> MSFTNATFSQVLDDLSARFILNLPAEEQSSVERLCFQIEQAHWFYEDFIRAQNDQLPSLGLRVFSAKLFAHCPLLWKWSKVHEEAFDDFLRYKTRIPVRGAIMLDMSMQQCVLVKGWKASSGWGFPKGKIDKDESDVDCAIREVYEETGFDCS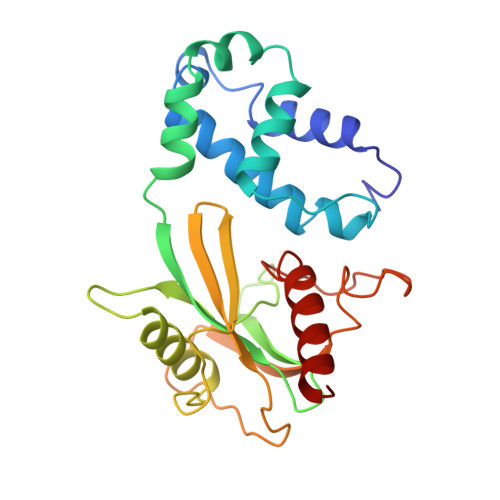SRINPNEFIDMTIRGQNVRLYIIPGISLDTRFESRTRKEISKIEWHNLMDLPTFKKNKPQTMKNKFYMVIPFLAPLKKWIKKRNIANNT3-(3-fluorophenyl)-N-{2-[2-(5-methyl-1H-imidazol-1-yl)pyrimidin-4-yl]ethyl}propan-1-amine | C19 H22 F 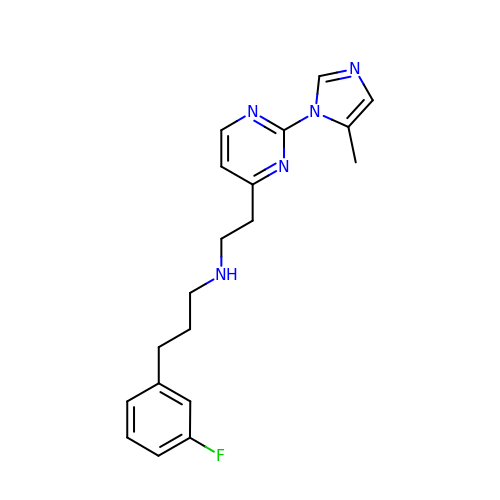N5 | XNNXUOKGLOGLRV-UHFFFAOYSA-N>DNVITRVVAVRNVSVRELSPLLRQLIDNAGAGNVVHYDPANIILITGRAAVVNRLAEIIKRVDQAGNREIEVVELGNASAAEMVRIVDALNRTTDAKNTPEFLQPKLVADERTNSILISGDPKVRDRLKRLIRQLDVEMASKGNNRVVYLKYAKAEDLVDVLKGVSDNLQAEKNSGQKGASSQRNDVVIAAHQGTNSLVLTAPPDIMLALQEVITQLDIRRAQVLIEALIVEMAEGDGVNLGVQWGNLETGAVIQYSNTGTPIGKVMVGLEEAKDKTVTDSRWNSDTDKYEPYSRTEAGDYSTLAAALAGVNGAAMSLVMGDWTALISAVSSDSNSNILSSPSITVMDNGEASFIVGEEVPVITGSTAGSNNDNPFQTVDRKEVGIKLKVVPQINEGDSVQLNIEQEVSNVLGANGAVDVRFAKRQLNTSVIVQDGQMLVLGGLIDERALESESKVPLLGDIPILGHLFKSTNTQVEKKNLMVFIKPTIIRDGMTADGITQRKYNYIRAEQLYKAEQGLKLMDDGHIPVLPKFGEDKRHPAEIQAFIDQMEQQ[15x]

Pathogenic bacteria commonly employ the Type II Secretion System (T2SS) for the release of protein toxins. The system includes an inner membrane platform of GspC-E-F-L-M, a periplasmic pseudopilus composed of GspG-H-I-J-K and the outer membrane secretion channel GspD, called the secretin. In numerous species the targeting, assembly and stability of the T2SS secretin in the outer membrane require the function of a small lipoprotein that binds to its C-terminal region (the S-domain) and serves to pilot secretin monomers from the inner to the outer membrane via the LOL lipoprotein sorting pathway. In this study we used cryo-electron microscopy to characterize the structure of the secretins from V. vulnificus and A. hydrophila and in addition determined the crystal structure of EpsS from V. vulnificus.

In addition, we also solved the cryo-EM structure of the EpsD secretin of V. vulnificus, which encodes both an EpsAB fusion and a GspSβ/AspS pilotin (EpsS). Analyses of top views of class averages revealed that, for both secretins, symmetry is unambiguously pentadecameric (C15 symmetry). The resolutions of the resulting symmetrized maps were estimated to be in the range of 3.4 Å for EpsD and 3.7 Å for ExeD by employing the gold standard FSC criterion. One of the clearest differences between the two types of secretins lies in the outermost region that is positioned towards the exterior of the cell. In EpsD this region is covered by a ‘cap’, formed by 15 aligned β-hairpins that lie on top of the membrane-embedded region. This region points towards the inside of the pore, closing the structure on the top. V. vulnificus EpsD, however, displays a well folded S-domain (residues 588–649) with a clear α-12. The Ala-Phe motif is present in EpsD, much as in its counterparts from V. cholerae and ETEC. Interestingly, as in the case of GspD, α-12 from the S-domain of EpsD was in a conformation that did not allow for EpsS binding, and our attempts to fit EpsS into this region led to clear clashes.> DPMAPPVRYCIPGERLCNLEEGSPGS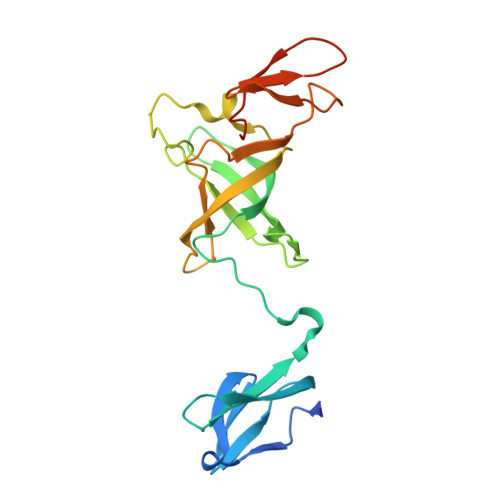GTYTRHGYIFSSLAGCLMKSSENGALPVVSVVRETESQLLPDVGAIVTCKVSSINSRFAKVHILYVGSMPLKNSFRGTIRKEDVRATEKDKVEIYKSFRPGDIVLAKVISLGDAQSNYLLTTAENELGVVVAHSESGIQMVPISWCEMQCPKTHTKEFRKVARVQPEFLQT> ETGSAKVAFSAIRSTNHEPSEMSNRTMIIYFDQVLVNIGNNFDSERSTFIAPRKGIYSFNFHVVKVYNRQTIQVSLMLNGWPVIS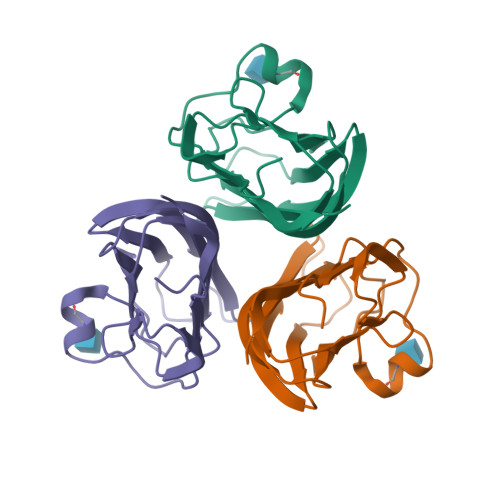AFAGDQDVTREAASNGVLIQMEKGDRAYLKLERGNLMGGWKYSTFSGFLVFPLGTKHHHHHH> MFFSQVLRSSARAAPIKRYTGGRIGESWVITEGRRLIPEIFQWSA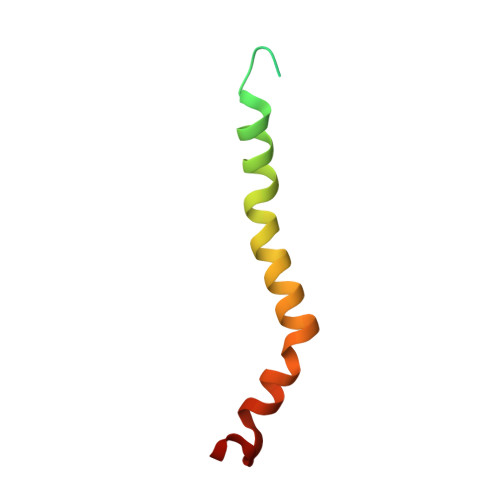VLSVCLGWPGAVYFFSKARKA> MSETSRTAFGGRRAVPPNNSNAAEDDLPTVELQGVVPRGVNLQEFLNVTSVHLFKERWDTNKVDHHTDKYENNKLIVRRGQSFYVQIDFSRPYDPRRDLFRVEYVIGRYPQENKGTYIPVPIVSELQSGKWGAKIVMREDRSVRLSIQSSPKCIVGKFRMYVAVWTPYGVLRTSRNPETDTYILFNPWCEDDAVYLDNEKEREEYVLNDIGVIFYGEVNDIKTRSWSYGQFEDGILDTCLYVMDRAQMDLSGRGNPIKVSRVGSAMVNAKDDEGVLVGSWDNIYAYGVPPSAWTGSVDILLEYRSSENPVRYGQCWVFAGVFNTFLRCLGIPARIVTNYFSAHDNDANLQMDIFLEEDGNVN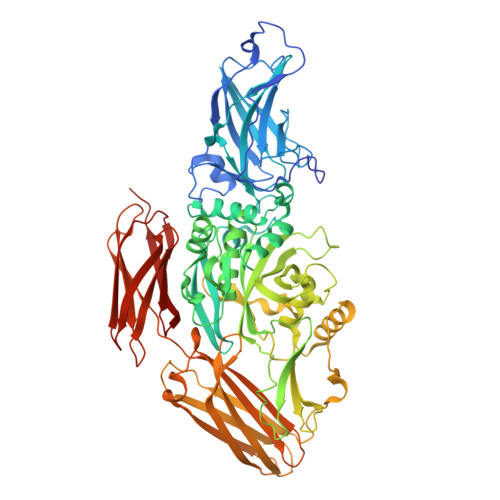SKLTKDSVWNYHCWNEAWMTRPDLPVGFGGWQAVDSTPQENSDGMYRCGPASVQAIKHGHVCFQFDAPFVFAEVNSDLIYITAKKDGTHVVENVDATHIGKLIVTKQIGGDGMMDITDTYKFQEGQEEERLALETALMYGAKKPLNTEGVMKSRSNVDMDFEVENAVLGKDFKLSITFRNNSHNRYTITAYLSANITFYTGVPKAEFKKETFDVTLEPLSFKKEAVLIQAGEYMGQLLEQASLHFFVTARINETRDVLAKQKSTVLTIPEIIIKVRGTQVVGSDMTVTVEFTNPLKETLRNVWVHLDGPGVTRPMKKMFREIRPNSTVQWEEVCRPWVSGHRKLIASMSSDSLRHVYGELDVQIQRRPSM>[7x]MTKINWEKYKKVIKKEFSEKEETEEVKNYIFSSQLDKVNLILEHMDTVGGIHSRNIAITGDRGTGKTSFIETLKLVLEKQNYYVFDIVSPTVLSSHL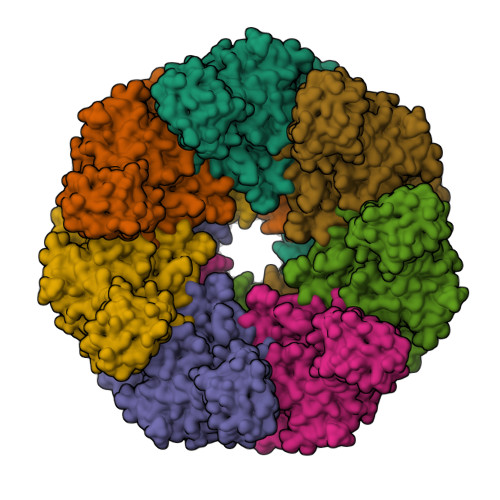NILEIVISSIYREIDQFIDSHDVHDRGRLIQHLKKVMNAIAVEKKQSDYFKQSKPEIEMLTDLSHRTFLDEEIKELFCYFKKVLNNRQDSCKEVIKDLVLIIDDLDLVENNLVYDLLRDIQHYLDSQLIVIFAYKEGQLEQSMFEHLAKGNEALLNHGVIDSNAIFGQIERFLTKLVPLSNRIPLFKQDELLNKTIGEFLASLDPSYGVGENLEFITKDSEKNKNNLTIREWFYESIFYRTNLKLDPIDIREEASRLMPKTLREMVQLCEELHSMQVITRSMDKLAGVEGLRKNIGAFRRYIGYKNSTYFNLATMEFFQKWELAESHQANYLAYHFLMSYYQESFEQNQKLGYPLNLSKSGYPLTLRTMEPYNITLGDIYALMEELKYTEGISADTYYIVYILKVYYSLRLSELLYNVVLHHKLFVHVKEEATTFYMATSTEELQIEKNHEQEATKLTDKEYREHIMTAIEKVPALQAYLELVNAQFMPQNFNYDRSGSRDDDFYLISWLKDDDLPEYSRLFKSLFLNSEVAAKGQIQRNIGKRESVFRYRNLYSYLPLQLTSATFYKIDFLAFAIKADLLMYNVVRFVEEEGDTIPYFMSNMFHIDVFVRHNYNENNNKGKFAYIAKQIVFGLWQGSNQRAHDLKHWYKSFDTVFGTKIEALHLLVDIAEQIKISDKQTTDVSALSEEQKRDEQAKKVAEKLAAIYHHIGMSRILSRLHQLPFIAEIKSNKELLQHFSEAIVKLEKYASDTINVGNLSQFRESLKKIGQTYPSIQVLVDKLHRKQKLYVEFIQDFIETVNKLGEADESN Galectin-8 is a member of the tandem-repeat galectin category, having two CRDs in tandem that are joined by an amino acid linker of variable length. The two CRDs of galectin-8, i.e. galectin-8N and galectin-8C, share ~40% sequence identity and exhibit differential glycan binding specificities. The galectin-8N CRD exhibits a typical β-sandwich comprising two anti-parallel β-sheets with the concave side housing the carbohydrate-binding site. The binding groove is formed from six beta strands labelled S1 to S6, with amino acids on strand S4-S6 forming the glycan recognition pocket (referred to as the “primary binding site”).

The galectin-8N-LNnT complex was obtained by soaking LNnT into an apo-crystal, and the structure was determined at 2.0 Å. The electron density maps showed unambiguous electron density for all the four sugars of the tetrasaccharide, and with the reducing end occupying the primary binding site. The lactose portion of LNnT retains the interactions observed previously in the galectin-8N-lactose complex. The other two sugars of LNnT extend through a β1-3 linkage into the extended binding site of galectin-8N contacting residues on strand S3 and S2. Due to the β1–4 linkage within the non-reducing end disaccharide (type 2 core), as opposed to the β1-3 linkage in LNT, all the four LNnT sugars stay close to the protein surface and interact with both the primary and the extended binding sites. The O6 of GlcNAc interacts with Gln47 and Asp49 and O3 is pointing away from the binding site into the solvent. The non-reducing end galactose ring forms CH-π type interactions with Tyr141 and O2 engages in hydrogen bonding interactions with Asp49. Despite having identical ligand conformation, the orientation of unique Arg59 on the long S3-S4 loop is different in our galectin-8N-LNnT complex to that seen in all the reported galectin-8N apo and ligand-bound structures. In the galectin-8N-LNnT complex, Arg59 is directed towards the non-reducing end galactose, whereas in the other structures, including the galectin-8N-LNFIII complex, it faces towards the conserved Trp86. Overall, the conformation of the LNnT core of LNFIII in the galectin-8N-LNFIII complex, is identical to that observed in our galectin-8N-LNnT-complex.

> MMLSLNNLQNIIYNPVIPFVGTIPDQLDPGTLIVIRGHVPSDADRFQVDLQNGSSVKPRADVAFHFNPRFKRAGCIVCNTLINEKWGREEITYDTPFKREKSFEIVIMVLKDKFQVAVNGKHTLLYGHRIGPEKIDTLGIYGKVNIHSIGFSFSS>[4x]MKFTPPPASLRNPLIIPEKIMMGPGPSNCSKRVLTAMTNTVLSNFHAELFRTMDEVKDGLRYIFQTENRATMCVSGSAHAGMEAMLSNLLEEGDRVLIAVNGIWAERAVEMSERYGADVRTIEGPPDRPFSLETLARAIELHQPKCLFLTHGDSSSGLLQPLEGVGQICHQHDCLLIVDAVASLCGVPFYMDKWEIDAVYTGAQKVLGAPPGITPISISPKALDVIRNRRTKS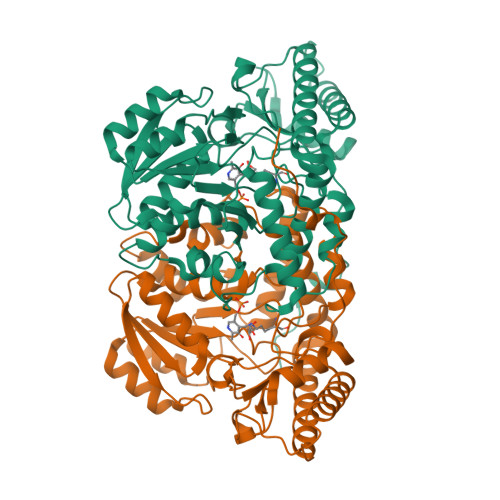KVFYWDLLLLGNYWGCYDEPKRYHHTVASNLIFALREALAQIAEEGLENQIKRRIECAQILYEGLGKMGLDIFVKDPRHRLPTVTGIMIPKGVDWWKVSQYAMNNFSLEVQGGLGPTFGKAWRVGIMGECSTVQKIQFYLYGFKESLKATHPDYIFEESNGFH> ERSSNNFNYGAYHSLEAIYHEMDNIAADFPDLARRVKIGHSFENRPMYVLKFSTGKGVRRPAVWLNAGIHSREWISQATAIWTARKIVSDYQRDPAITSILEKMDIFLLPVANPDGYVYTQTQNRLWRKTRSRNPGSSCIGADPNRNWNASFAGKGASDNPCSEVYHGPHANSEVEVKSVVDFIQKHGNFKGFIDLHSYSQLLMYPYGYSVKKAPDAEELDKVARLAAKALASVSGTEYQVGPTCTTVYPASGSSIDWAYDNGIKFAFTFELRD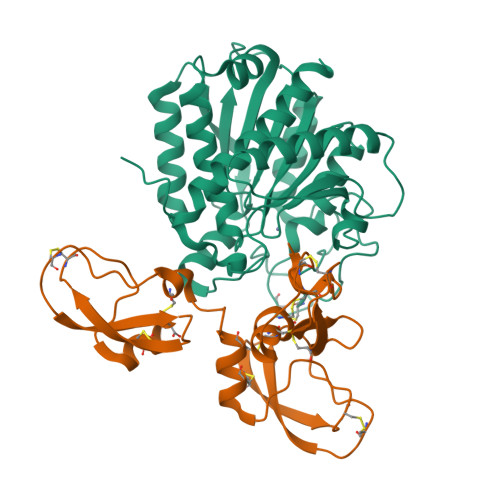TGTYGFLLPANQIIPTAEETWLGLKTIMEHVRDNLY;> ISVCDLPADRGQCTAYIPQWFFAKTTEDCEKFVYGGCQGNANRFETKDDCIANCGCNLPSKVGPCRVSARMWFHNPETEKCEVFIYGGCHGNANRFATETECQEVCDRYQKPGFCYQPSETGPCKGSFPRYYYDYEDGECKEFIYGGCEGNANNFETKESCENAC>[6x]MKTVVFAYHDMGCLGIEALLAAGYEISAIFTHTDNPGEKAFYGSVARLAAERGIPVYAPDNVNHPLWVERIAQLSPDVIFSFYYRHLIYDEILQLAPAGAFNLHGSLLPKYRGRAPLNWVLVNGETETGVTLHRMVKRAD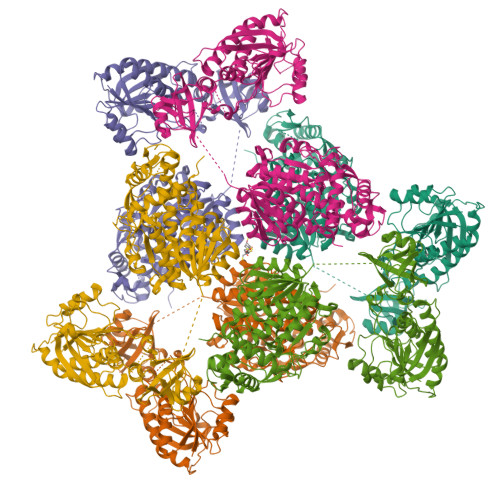AGAIVAQLRIAIAPDDIAITLHHKLCHAARQLLEQTLPAIKHGNILEIAQRENEATCFGRRTPDDSFLEWHKPASVLHNMVRAVADPWPGAFSYVGNQKFTVWSSRVHPHASKAQPGSVISVAPLLIACGDGALEIVTGQAGDGITMQGSQLAQTLGLVQGSRLNSQPACTARRRTRVLILGVNGFIGNHLTERLLREDHYEVYGLDIGSDAISRFLNHPHFHFVEGDISIHSEWIEYHVKKCDVVLPLVAIATPIEYTRNPLRVFELDFEENLRIIRYCVKYRKRIIFPSTSEVYGMCSDKYFDEDHSNLIVGPVNKPRWIYSVSKQLLDRVIWAYGEKEGLQFTLFRPFNWMGPRLDNLNAARIGSSRAITQLILNLVEGSPIKLIDGGKQKRCFTDIRDGIEALYRIIENAGNRCDGEIINIGNPENEASIEELGEMLLASFEKHPLRHHFPPFAGFRVVESSSYYGKGYQDVEHRKPSIRNAHRCLDWEPKIDMQETIDETLDFFLRTVDLTDKPS> MQIGFNFTLTGTLDMVQQMIKERKIDYVEMLIDNFVHLPPEQIADSFDC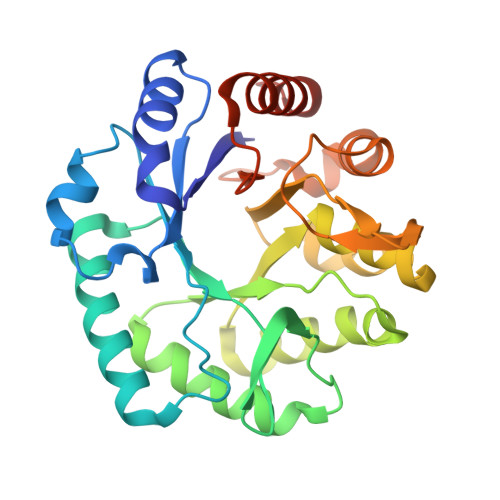PVAFHIMLSKYLERDREALAALGKRLRRFIDVMRPVYVSDHILYFTHNGRSLFHLGEIDYGEYDHVRSKVEQWQDMLGTRLYLENYPSIMDGAWDAPSFYERLSRETGVGVLFDASNAICAQNNTGAPVELWKKIIETTRHFHVAGYGTAFIEPRVKADTHDREMAEDTLDFLSRMRTSFDKPGATITYERDFDIDYESISVDLKRLRDIFPCVEEERH> GSHMATPPKRSCPSFSASSEGTRIKKISIEGNIAAGKSTFVNILKQLCEDWEVVPEPVARWCNVQSTQDEFEELTMSQKNGGNVLQMMYEKPERWSFTFQTYACLSRIRAQLASLNGKLKDAEKPVLFFERSVYSDRYIFASNLYESECMNETEWTIYQDWHDWMNNQFGQSLELDGIIYLQATPETCLHRIYLRGRNEEQGIPLEYLEKLHYKHESWLLHRTLKT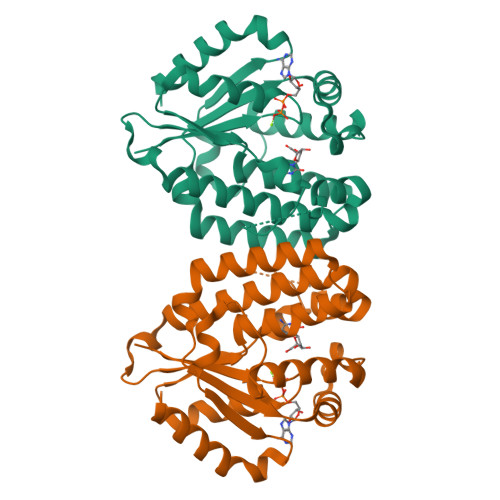NFDYLQEVPILTLDVNEDFKDKYESLVEKVKEFLSTL> LEVPKHMRSGAKKLTNLCIKETGVTEDLFIEAQETGKMPNNQRLKCFIHCVLDKIGLIDADNIVHLDNLLEILPPEFVPIVEELHTTCGTQSGADGCETAFLTTECYIKTNPVILKL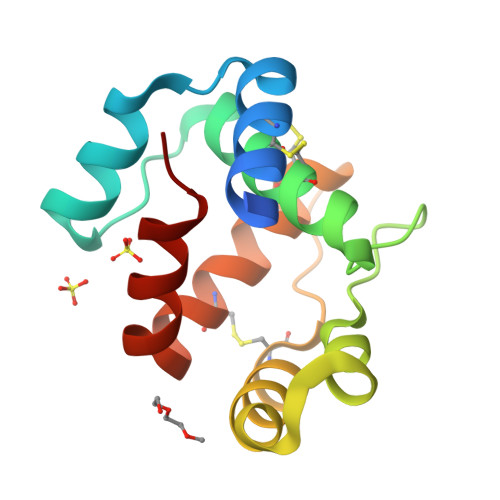LFTTFSE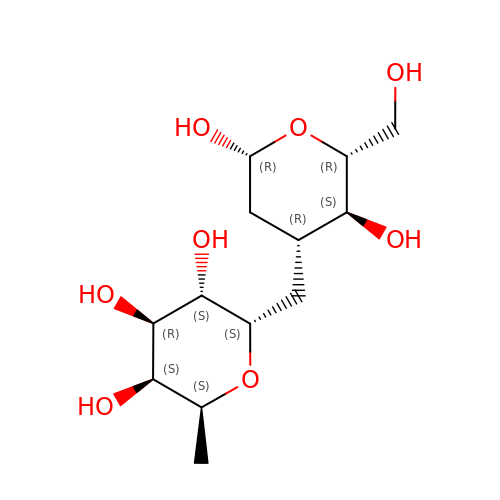(2~{S},3~{S},4~{R},5~{S},6~{S})-2-[[(2~{R},3~{S},4~{R},6~{R})-2-(hydroxymethyl)-3,6-bis(oxidanyl)oxan-4-yl]methyl]-6-methyl-oxane-3,4,5-triol | C13 H24 O8 | DUFGPMLQNGKXRP-CRMQZNGFSA-N>SMIKQRTLKNIIRATGVGLHSGEKVYLTLKPAPVDTGIVFSRTDLDPVVEIPARAENVGETTMSTTLVKGDVKVDTVEHLLSAMAGLGIDNAYVELSASEVPIMDGSAGPFVFLIQSAGLQEQEAAKKFIRIKREVSVEEGDKRAVFVPFDGFKVSFEIDFDHPVFRGRTQQASVDFSSTSFVKEVSRARTFGFMRDIEYLRSQNLALGGSVENAIVVDENRVLNEDGLRYEDEFVKHKILDAIGDLYLLGNSLIGEFRGFKSGHALNNQLLRTLIADKDAWEV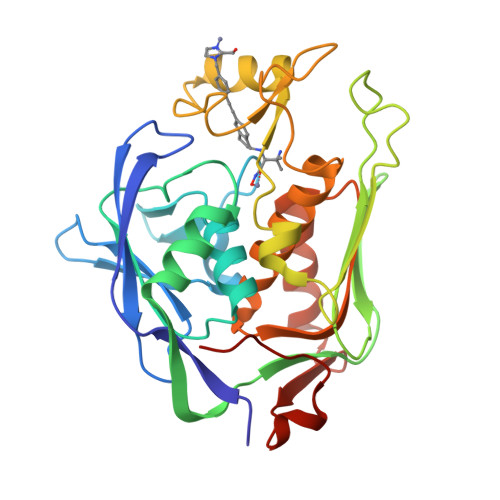VTFEDARTAPISYMRPAAAV[2x]> GPLGSLFRSLVGTSRAIQQVRQMMQQVADTDASVLILGESGTGKEVVARNLHYHSKRREGPFV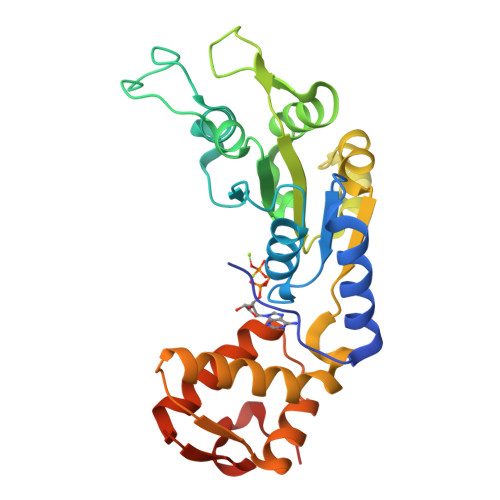PVNCGAIPAELLESELFGHEKGAFTGAITSRAGRFELANGGTLFLDEIGDMPLPMQVKLLRVLQERTFERVGSNKTQNVDVRIIAATNKNLEKMIEDGTFREDLYYRLNVFPIEMAPLRERVEDIALLLNELISRMEHEKRGSIRFNSAAIMSLCRHDWPGNVRELANLVERLAIMHPYGVIGVGELPKKFRHVDDEDEQ In this study, we extracted extracellular fibrils from lab-cultured Bacillus amyloiquefaciens, a Gram-positive bacterium with great potential in biotechnological applications such as plant growth promotion, biocontrol, and commercial enzyme production. In this study, we use cryo-EM to identify protein fibrils surrounding lab-cultured Bacillus amyloiquefaciens and discover an unreported fibril species in addition to the flagellar fibrils. In summary, our study identified two protein fibrils outside Bacillus bacteria: the extensively studied flagella and the previously undiscovered Vpr fibrils.

The first fibril species was identified to be flagellar fibrils due to the similarities of its 2D classes and 3D map to that of Bacillus subtilis flagella. Upon structural comparison, we observed differences between Bacillus amyloiquefaciens and Bacillus subtilis flagella, namely: (1) the former contains an additional D2 domain, whereas the later contains only D0 and D1 domains; (2) the later has three additional loops (L1, L2, and L3) compared to the former. These differences arise from the sequence variations between the two proteins (sequence identity 57%). Notably, these variable regions face outward from the flagellar fibrils and do not affect the assembly of flagella. In summary, our findings suggest that while the structures of flagella in Bacillus amyloiquefaciens and Bacillus subtilis are largely conservative, there are notable differences in their domain compositions that likely reflect sequence variations between the two proteins.

>MRINHNIAALNTSRQLNAGSNAASKNMEKLSSGLRINRAGDDAAGLAISEKMRSQIRGLDMASKNAQDGISLIQTSEGALNETHSILQRMSELATQAANDTNTDSDRSELQKEMDQLASEVTRISTDTEFNTKKLLDGTAQNLTFQIGANEGQTMSLSINKMDSESLKVGTTYTANDDGSKLVTADGKEATLVTDGSKGPNGYYDDADKLVYQADSALAKDTKVTKGIDISSSAKAASSALTTIKTAIDTVSSERAKLGAVQNRLEHTINNLGTSSENLTSAESRIRDVDMASEMMEYTKNNILTQASQAMLAQANQQPQQVLQLLKG[33x]7-({4-[(3R)-3-aminopyrrolidin-1-yl]-5-chloro-6-ethyl-7H-pyrrolo[2,3-d]pyrimidin-2-yl}sulfanyl)pyrido[2,3-b]pyrazin-2(1H)-one 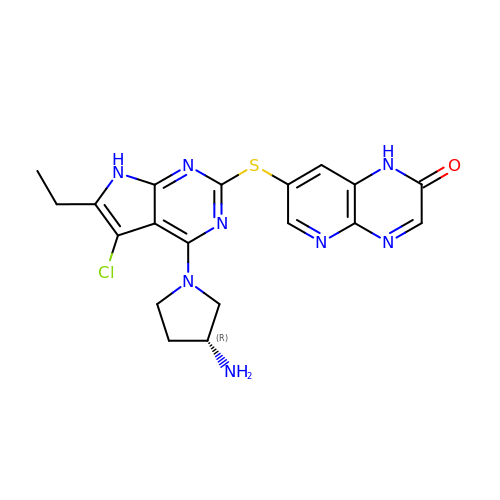| C19 H19 Cl N8 O S | QARZTJJXVNQVNZ-SECBINFHSA-N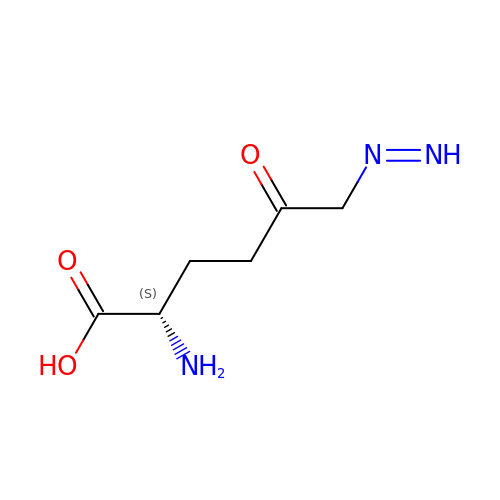6-DIAZENYL-5-OXO-L-NORLEUCINE | C6 H11 N3 O3 | CKRLZVNSTCQAJW-YFKPBYRVSA-N> DAAQPARRARRTYEAYPAKPKCPAVCTCTKDNALCENARSIPRTVPPDVISLSFVRSGFTEISEGSFLFTPSLQLLLFTSNSFDVISDDAFIGLPHLEYLFIENNNIKSISRHTFRGLKSLIHLSLANNNLQTLPKDIFKGLDSLTNVDLRGNSFNCDCKLKWLVEWLGHTNATVEDIYCEGPPEYKKRKINSLSSKDFDCIIKHHHHHH

LGI1 is a 60-kDa secreted neuronal protein, which consists of the N-terminal leucine-rich repeat (LRR) domain and the C-terminal epitempin-repeat (EPTP) (also known as EAR) domain4. ADAM22 serves as a receptor for LGI1 and is anchored to the excitatory postsynaptic density through PSD-95 scaffold. The LGI1–ADAM22 ligand–receptor interaction plays an essential role in AMPA-type glutamate receptor-mediated synaptic transmission via PSD-9533–35. In this study, we present the crystal structures of LGI1 LRR, LGI1 EPTP–ADAM22, and LGI1–ADAM22 at 1.78, 2.67, and 7.13 Å resolutions, respectively.

For this mapping, we also determined the crystal structure of LGI1 LRR alone at 1.78 Å resolution. Correspondingly, the C42R, C42G, C46R, C46F, C179R, and C200R mutations disrupt intramolecular disulfide bonds in the N- and C-terminal caps of LGI1 LRR, which are common in extracellular and membrane-associated LRR proteins to stabilize their N- and C-terminal edges. However, we suspected that the trimer-of-dimer assembly seems unlikely because LGI1 LRR and LGI1 EPTP–ADAM22 themselves exhibit no obvious structural features suggestive of trimer formation.>GHMAKRVFFSFHYQDVIDFRVNVVRNHWVTKLNQSAAGVFDASLWEDAKKTSDIALKRLINGGLNNTSVTCVLIGSQTFNRRWVRYEIMKSIEKGNKIIGIHINAFKDKYGNIKSKGPNPFDYLGYQYSSDGKQLHLYEWTGGKWEEYKDLAPYRVNQIAPESLRGKFYSLSSVYRVYD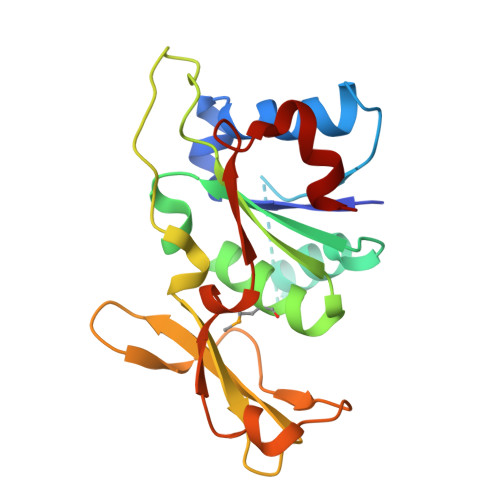WVADDGYNKFSSWVN[2x]>MPLFNSILDTIGRTPIVRLQRMAPEHTSVYVKVESFNPGGSVADRLALSVVLDAEAKGLLKPGDTIVECTSGNVGIALAMVAAARGYRFVAVMGDTYSVERRKLIRAYGGKLVLFPGHLGSKGGNLIADELAEKYGWFRARQFDNPANPSYHRETTASEILADFAGKRLDHFVTGFGTTGTLTGVGQMLRVARPEVRVVALEPSNAAMLARGEWSPHQIQGLAPNFVPGVLDRSVIDDLVTMDEVTARDTSRRLAAEEGIFAGISAGATVATALSIAEHAPEGTVLLAMLPDTGERYLSTFLFDGVDEGSDDAWLASLDTGSGLLEHHHHHH[2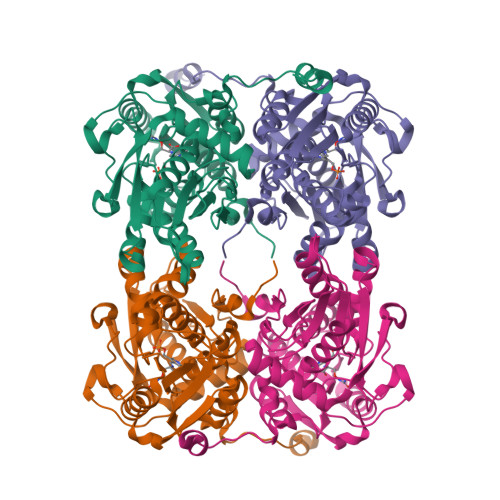x]IODOETHANE | C2 H5 I 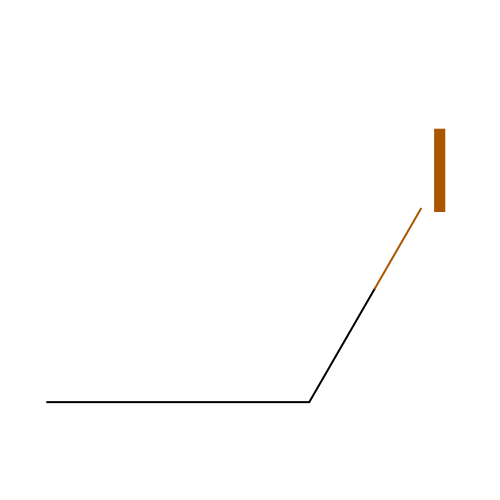| HVTICUPFWKNHNG-UHFFFAOYSA-N> GGGHNVAWDYDNNVIRGVNLGGWFVLQPYMTPSLFEPFQNGNDQSGVPVDEYHWTQTLGKEAALRILQKHWSTWITEQDFKQISNLGLNFVRIPIGYWAFQLLDNDPYVQGQVQYLEKALGWARKNNIRVWIDLHGAPGSQNGFDNSGLRDSYNFQNGDNTQVTLNVLNTIFKKYGGNEYSDVVIGIELLNEPLGPVLNMDKLKQFFLDGYNSLRQTGSVTPVIIHDAFQVFGYWNNFLTVAEGQWNVVVDHHHYQVFSGGELSRNINDHISVACNWGWDAKKESHWNVAGEWSAALTDCAKWLNGVNRGARYEGAYDNAPYIGSCQPLLDISQWSDEHKTDTRRYIEAQLDAFEYTGGWVFWSWKTENAPEWSFQT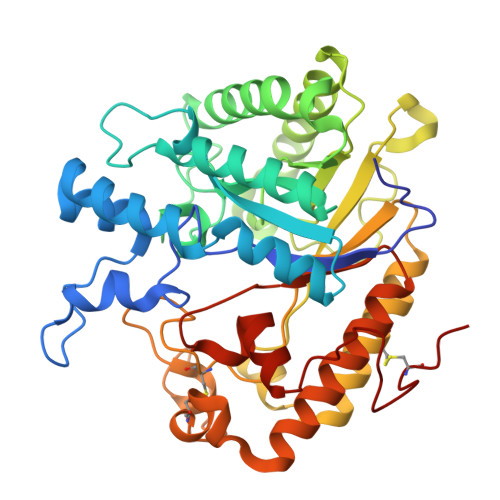LTYNGLFPQPVTDRQFPNQCGFH> GAMCYIIA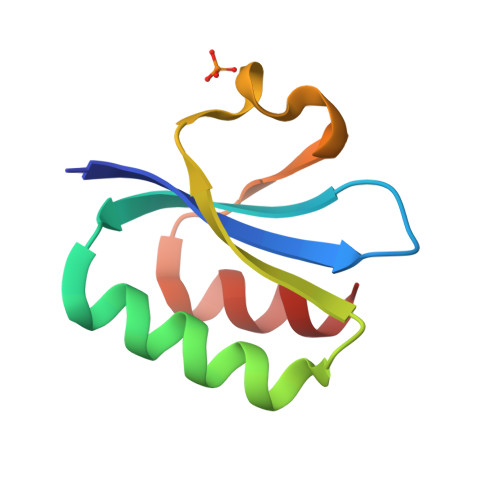KRFKKSGCVALKAKRGKELADFATDLQKKLGYDIQIVAITRPTAYGEYEPYKFVNSFEEFSIEASRL> AMRQCAIYGKGGIGKSTTTQNLVAALAEMGKKVMIVGCDPKADSTRLILHSKAQNTIMEMA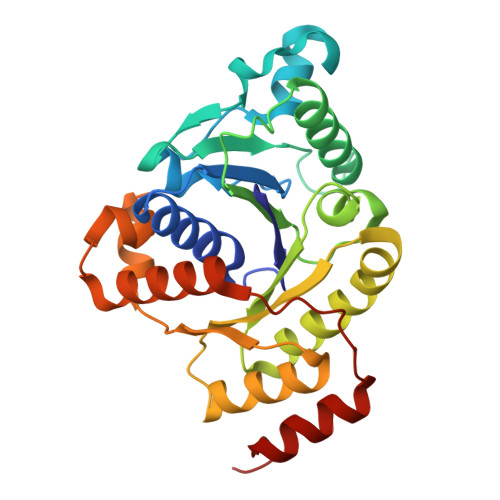AEAGTVEDLELEDVLKAGYGGVKCVESGGPEPGVGCAGRGVITAINFLEEEGAYEDDLDFVFYDVLGDVVCGGFAMPIRENKAQEIYIVCSGEMMAMYAANNISKGIVKYANSGSVRLGGLICNSRNTDREDELIIALANKLGTQMIHFVPRDNVVQRAEIRRMTVIEYDPKAKQADEYRALARKVVDNKLLVIPNPITMDELEELLMEFGIMEV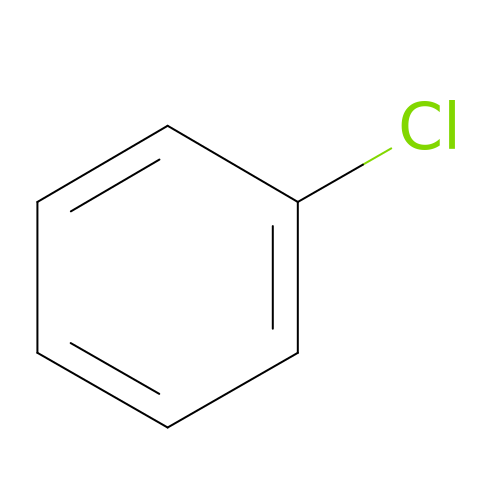chlorobenzene | C6 H5 Cl | MVPPADPHJFYWMZ-UHFFFAOYSA-N>[2x]MASTKAPGPGEKHHSIDAQLRQLVPGKVSEDDKLIEYDALLVDRFLNILQDLHGPSLREFVQECYEVSADYEGKGDTTKLGELGAKLTGLAPADAILVASSILHMLNLANLAEEVQIAHRRRNSKLKKGGFADEGSATTESDIEETLKRLVSEVGKSPEEVFEALKNQTVDLVFTAHPTQSARRSLLQKNARIRNCLTQLNAKDITDDDKQELDEALQREIQAAFRTDEIRRAQPTPQAEMRYGMSYIHETVWKGVPKFLRRVDTALKNIGINERLPYNVSLIRFSSWMGGDRDGNPRVTPEVTRDVCLLARMMAANLYIDQIEELMFELSMWRCNDELRVRAEELHSSSGSK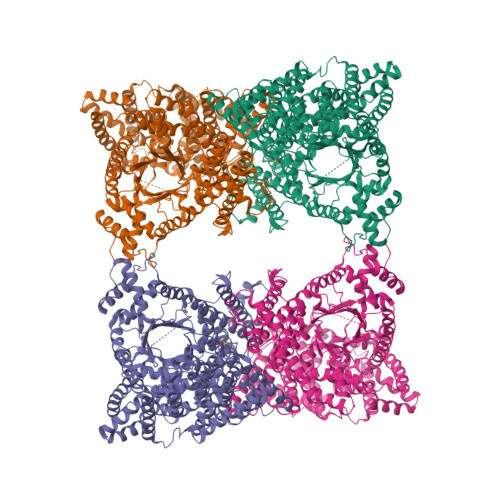VTKYYIEFWKQIPPNEPYRVILGHVRDKLYNTRERARHLLASGVSEISAESSFTSIEEFLEPLELCYKSLCDCGDKAIADGSLLDLLRQVFTFGLSLVKLDIRQESERHTDVIDAITTHLGIGSYREWPEDKRQEWLLSELRGKRPLLPPDLPQTDEIADVIGAFHVLAELPPDSFGPYIISMATAPSDVLAVELLQRECGVRQPLPVVPLFERLADLQSAPASVERLFSVDWYMDRIKGKQQVMVGYSDSGKDAGRLSAAWQLYRAQEEMAQVAKRYGVKLTLFHGRGGTVGRGGGPTHLAILSQPPDTINGSIRVTVQGEVIEFCFGEEHLCFQTLQRFTAATLEHGMHPPVSPKPEWRKLMDEMAVVATEEYRSVVVKEARFVEYFRSATPETEYGRMNIGSRPAKRRPGGGITTLRAIPWIFSWTQTRFHLPVWLGVGAAFKFAIDKDVRNFQVLKEMYNEWPFFRVTLDLLEMVFAKGDPGIAGLYDELLVAEELKPFGKQLRDKYVETQQLLLQIAGHKDILEGDPFLKQGLVLRNPYITTLNVFQAYTLKRIRDPNFKVTPQPPLSKEFADENKPAGLVKLNPASEYPPGLEDTLILTMKGIAAGMQNTG> SNAGVSDVEL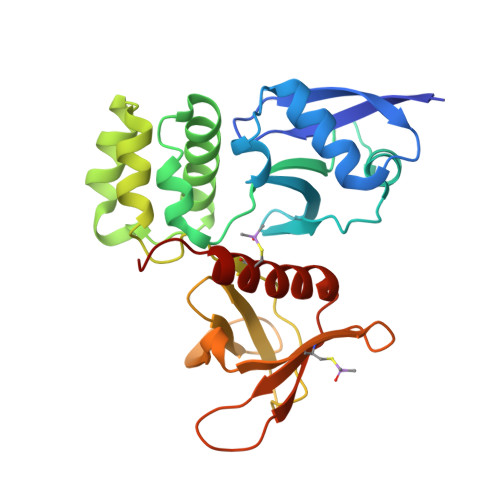RVALPDGTTVTVRVKKNSTTDQVYQAIAAKVGMDSTTVNYFALFEVISHSFVRKLAPNEFPHKLYIQNYTSAVPGTCLTIRKWLFTTEEEILLNDNDLAVTYFFHQAVDDVKKGYIKAEEKSYQLQKLYEQRKMVMYLNMLRTCEGYNEIIFPHCACDSRRKGHVITAISITHFKLHACTEEGQLENQVIAFEWDEMQRWDTDEEGMAFCFEYARGEKKPRWVKIFTPYFNYMHECFERVFCELKWRKEEY>[4x]MATQGVFTLPANTRF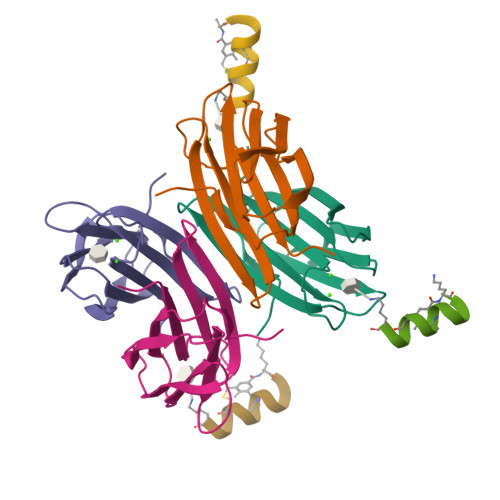GVTAFANSSGTQTVNVLVNNETAATFSGQSTNNAVIGTQVLNSGSSGKVQVQVSVNGRPSDLVSAQVILTNELNFALVGSEDGTDNDYNDAVVVINWPLG;>XKKLLKCLKCLLKX[3x]> MSQTSTLKGQCIAEFLGTGLLIFFGVGCVAALKVAGASFGQWEISVIFGLGVAMAIYLTAGVSGAHLNPAVTIALWLFACFDKRKVIPFIVSQVAG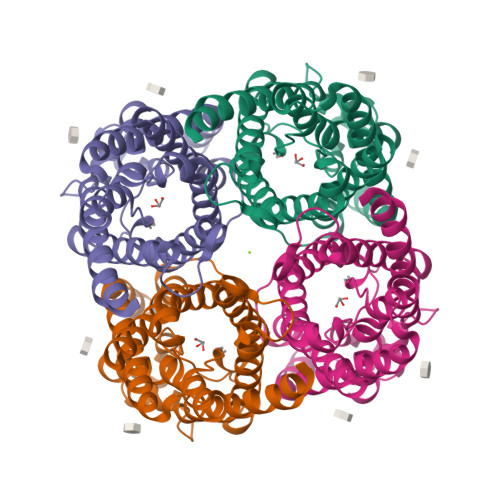AFCAAALVYGLYYNLFFDFEQTHHIVRGSVESVDLAGTFSTYPNPHINFVQAFAVEMVITAILMGLILALTDDGNGVPRGPLAPLLIGLLIAVIGASMGPLTGTAMNPARDFGPKVFAWLAGWGNVAFTGGRDIPYFLVPLFGPIVGAIVGAFAYRKLIGRHLPCDICVVEEKETTTPSEQKASL> QKDANFASGRNSIVHLFEWKWNDIADECERFLQPQGFGGVQISPPN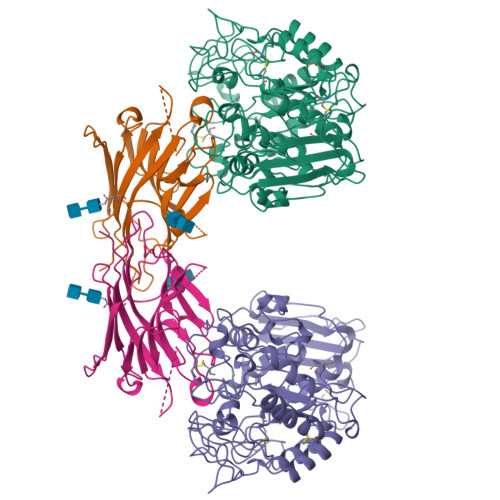EYLVADGRPWWERYQPVSYIINTRSGNESAFTDMTRRCNDAGVRIYVDAVINHMTGMNGVGTSGSSADHDGMNYPAVPYGSGDFHSPCEVNNYQDADNVRNCELVGLRDLNAGSDYVRGVLIDYMNHMIDLGVAGFRVDAAKHMSPGDLSVIFDGLKNLNTDYGFADGARPFIYQEVIDLGGEAISKNEYTGFGCVLEFQFGVSLGNAFQGGNQLKNLANWGPEWGLLEGLDAVVFVDNHDNQRTGGSQILTYKNPKPYKMAIAFMLAHPYGTTRIMSSFDFTDNDQGPPQDGSGNLISPGINDDNTCSNGYVCEHRWRQVYGMVGFRNAVEGTQVENWWSNDDNQIAFSRGSQGFVAFTNGGDLNQNLNTGLPAGTYCDVISGELSGGSCTGKSVTVGDNGSADISLGSAEDDGVLAIHVNAKL;> ATETSFIIDAFNKTNLILQGDATVSSNGNLQLSYNSYDSMSRAFYSAPIQIRDSTTGNVASFDTNFTMNIRTHRQANSAVGLDFVLVPVQPESKGDTVTVEFDTFLSRISIDVNNNDIKSVPWDVHDYDGQNAEVRITYNSSTKVFSVSLSNPSTGKSNNVSTTVELEKEVYDWVSVGFSATSGAYQWSYETHDVLSWSFSSKFI> M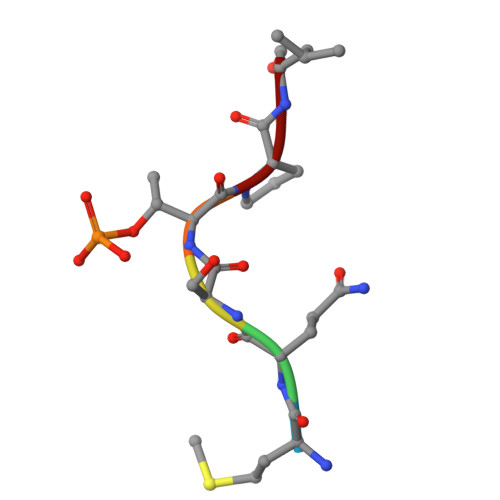QSTPL>[5x]MKGGAGVPDLPSLDASGVRLAIVASSWHGKICDALLDGARKVAAGCGLDDPTVVRVLGAIEIPVVAQELARNHDAVVALG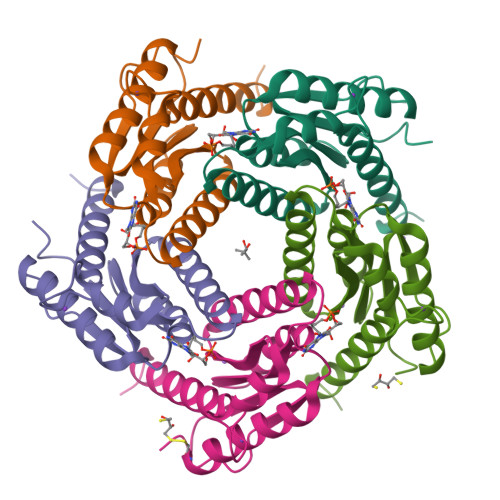VVIRGQTPHFDYVCDAVTQGLTRVSLDSSTPIANGVLTTNTEEQALDRAGLPTSAEDKGAQATVAALATALTLRELRAHS> MPKRIVYNISSDFQLKSL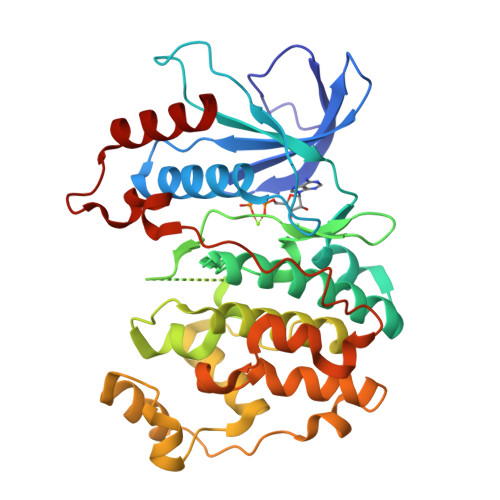LGEGAYGVVCSATHKPTGEIVAIKKIEPFDKPLFALRTLREIKILKHFKHENIITIFNIQRPDSFENFNEVYIIQELMQTDLHRVISTQMLSDDHIQYFIYQTLRAVKVLHGSNVIHRDLKPSNLLINSNCDLKVCDFGLARIIDESAADNSEPTGQQSGMTEYVATRWYRAPEVMLTSAKYSRAMDVWSCGCILAELFLRRPIFPGRDYRHQLLLIFGIIGTPHSDNDLRCIESPRAREYIKSLPMYPAAPLEKMFPRVNPKGIDLLQRMLVFDPAKRITAKEALEHPYLQTYHDPNDEPEGEPIPPSFFEFDHYKEALTTKDLKKLIWNEIFS>[2x]MGSSHHHHHHSSGLVPRGSHMASKRCRQCSGDSASSSTSSLSPSELPPSKKAAGGQRVTAEVEVAPITTDATSATVTAAGGAKKKATTGSPARRTSSAAKITNGDAGELIRTAEALAALNAKKSEKEIWSD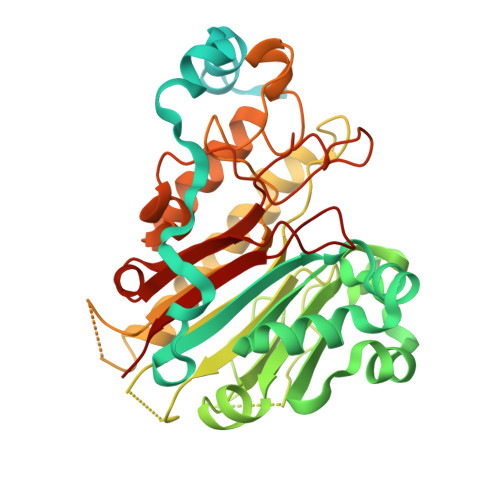VVPFVRRTTDSDFDPSRMYKFITWNVAGLRGLLKKNASALRAFMEAEKPDVLCLQETKLNVDEADANATLGVVDGYSFVDHPCAFKRGYSGTRTYMKNSTTVKGLHARCTRGFALPSEPQADAAAGSRVLVEGAGDEEGRVLTTFLSPDPDSASSSSRIALVNTYVANSGMGLTRLPYRVQSFDPSMREYLHRLDTWATENAAVPSAAAMGSGSSPHGFIWAGDLNVAERDYDRYYAGTFKSMQECSGFAPEERMSFRETMQRTNSVDIFRQLYPQAGPVYSFWSQRINGRPRNLGWRLDYFVVSSRLASYVVDCFPMPTVMGSDHCPFQMWMRHP Phosphoglycerate mutases (PGMs) catalyse the interconversion of 2- and 3-phosphoglycerate (2-PG; 3-PG) in the glycolytic and gluconeogenic pathways. The enzymes have no amino-acid sequence similarity and differ in their mechanism of catalysis. iPGM is comprised of ∼510 amino acids and facilitates the intramolecular transfer of the phosphoryl group on the monophosphoglycerates through a phosphoserine intermediate and is the sole PGM in nematode. The iPGMs are monomeric bi-domain enzymes where a phosphatase domain, structurally related to the alkaline phosphatase family of binuclear metalloenzymes, is connected by two hinge peptides to a phosphotransferase domain8. The glycolytic phosphoglycerate mutase, iPGM is an attractive target for the development of broad spectrum antiparasitic and antibacterial agents owing to its essential metabolic function and evolutionary divergence from the human enzyme.

In a subsequent crystallization effort, using an 18 amino-acid N-terminal truncated form of C. elegans iPGM, we prepared a pre-formed Ce-2 complex purified by sizing chromatography, as well as a mixture with Ce-2d. The latter resulted in needle-like crystals diffracting to 1.95 Å. The two subunits of the asymmetric unit are nearly identical with an RMSD of 0.20 Å between Cα atoms for 520 residues aligned. The cavity that accommodates the binding of the Ce-2d cyclic peptide is very similar amongst all of the structures with no marked conformational changes observed to accommodate binding of the peptide. A relatively small region of the total Ce-2d peptide surface makes direct contact to iPGM (127.1 Å2) with the remaining area (305 Å2) exposed to solvent as it is positioned within an open pocket between the phosphatase and transferase domains. The electron density for the cyclic peptide was prominent for all of the residues except for the terminal tyrosine side chain which was somewhat disordered, while the C-terminal 4 residues form a short α-helix. The three extra-cyclic C-terminal residues, Tyr9, Leu10 and Tyr11 are wrapped close to the core macrocycle, with the carboxamide of Tyr11 visible on the exterior surface of this compact structure and pointing toward the metal ion active site. Notably, the Ce-2d C-terminal amide of the Tyr11 residue is 6.5 and 8.4 Å from the Mn2+and Zn2+ ions, respectively. The model places the macrocycle at a site non-overlapping with phosphoglycerate supporting an allosteric binding mode for the ipglycermides.

>[2x]MAMANNSSVANKVCLIVIDGWGVSEDPYGNAILNAQTPVMDKLCSGNWAQIEAHGLHVGLPEGLMGNSEVGHLNIGAGRVIYQDIVRINLAVKNNKFVTNESLVDACDRAKNGNGRLHLAGLVSDGGVHSHIDHMFALVKAIKELGVPELYLHFYGDGRDTSPNSGVGFLEQTLEFLEKTTGYGKLATVVGRYYAMDRDNRWERINVAYEAMIGGVGETSDEAGVVEVVRKRYAADETDEFLKPIILQGEKGRVQNDDTIIFFDYRADRMREISAAMGMDRYKDCNSKLAHPSNLQVYGMTQYKAEFPFKSLFPPASNKNVLAEWLAEQKVSQFHCAETEKYAHVTFFFNGGLEKQFEGEERCLVPSPKVATYDLQPEMSAAGVADKMIEQLEAGTHPFIMCNFAPPDMVGHTGVYEAAVKACEATDIAIGRIYEATQKHGYSLMVTADHGNAEKMKAPDGGKHTAHTCYRVPLTLSHPGFKFVDPADRHPALCDVAPTVLAIMGLPQPAEMTGVSIVQKIKLAAALEHHHHHH;>[2x]XYDYPGDYCYLYX> SEVSDTNLYSPFKPRNYQLELALPAMKGKNTIICAPTGCGKTFVSLLICEHHLKKFPQGQKGKVVFFANQIPVYEQNKSVFSKYFERHGYRVTGISGATAENVPVEQIVENNDIIILTPQILVNNLKKGTIPSLSIFTLMIFDECHNTSKQHPYNMIMFNYL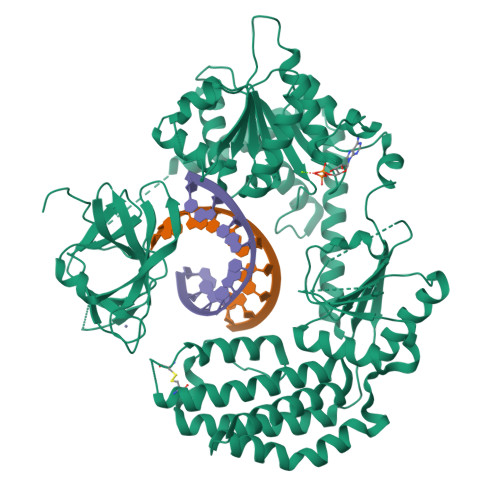DQKLGGSSGPLPQVIGLTASVGVGDAKNTDEALDYICKLCASLDASVIATVKHNLEELEQVVYKPQKFFRKVESRISDKFKYIIAQLMRDTESLAKRICKDLENLSQSQNREFGTQKYEQWIVTVQKACMVFQMPDKDEESRICKALFLYTSHLRKYNDALIISEHARMKDALDYLKDFFSNVRAAGFDEIEQDLTQRFEEKLQELESVSRDPSNENPKLEDLCFILQEEYHLNPETITILFVKTRALVDALKNWIEGNPKLSFLKPGILTGRGKTNQNTGMTLPAQKCILDAFKASGDHNILILTSVADEGIDIAQCNLVILYEYVGNVIKMIQTRGRGRARGSKCFLLTSNAGVIEKEQINMYKEKMMNDSILRLQTWDEAVFREKILHIQTHEKFIRDSQEKPKPVPDKENKKLLCRKCKALACYTADVRVIEDCHYTVLGDAFKECFVSRPHPKPKQFSSFEKRAKIFCARQNCSHDWGIHVKYKTFEIPVIKIESFVVEDIATGVQTLYSKWKDFHFEKIPFDPAEMSK>[2x]GSHMTEGTIKTSKYEIIAIFREELRKRTEIEIFFNNTSIITQLTRVD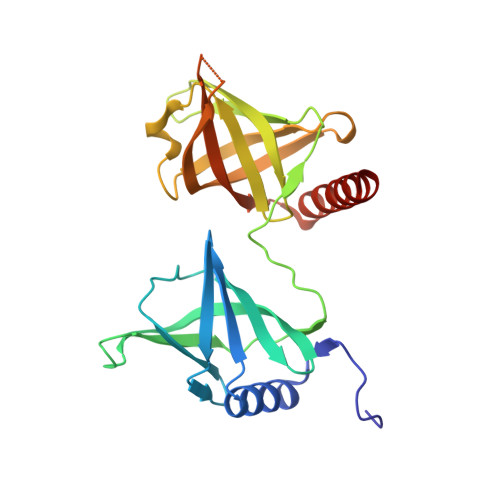FAEFHIQTHRKIPSGHKIRFLLHSDSGKIEFNAALTKHDNSGVDKGIRYAFSLPECLQVVQRRRDPRFRLRHEHDFYCRGRHKNGENYLFDIKDISDGGCALMTKTPNLKFLSHNALLKNAVLMLAEYGEITIDLVVKNVIVITLDNANEESESYYQISCQFKFRHLDDQRRIEKILLDLILEAKRKKRI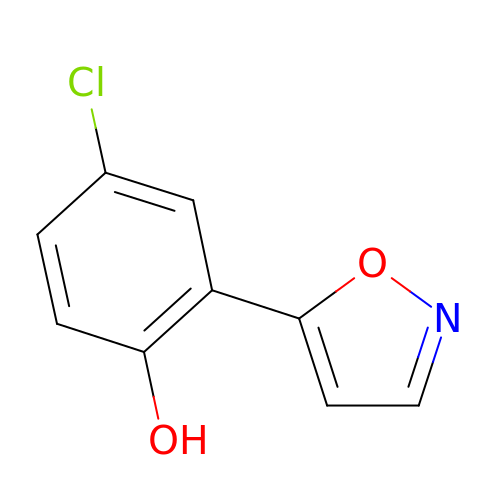4-chloro-2-isoxazol-5-yl-phenol | C9 H6 Cl N O2 | AAJXJLYUWKMQNO-UHFFFAOYSA-N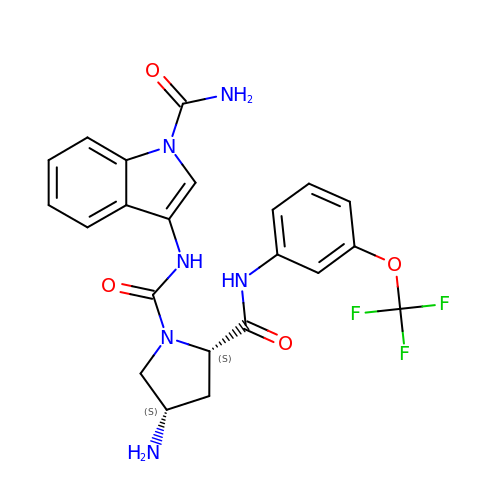(2~{S},4~{S})-~{N}1-(1-aminocarbonylindol-3-yl)-4-azanyl-~{N}2-[3-(trifluoromethyloxy)phenyl]pyrrolidine-1,2-dicarboxamide | C22 H21 F3 N6 O4 | BOUWILWEXWTKKH-SGTLLEGYSA-N> MISYDNYVTILDEETLKAWIAKLEKAPVFAFDTETDSLDNISANLVGLSFAIEPGVAAYIPVAHDYLDAPDQISRERALELLKPLLEDEKALKVGQNLKYDRGILANYGIELRGIAFDTMLESYILNSVAGRHDMDSLAERWLKHKTITFEEIAGKGKNQLTFNQIALEEAGRYAAEDADVTLQLHLKMWPDLQKHKGPLNVFENIEMPLVPVLSRIERNGVKIDPKVLHNHSEELTLRLAELEKKAHEIAGEEFNLSSTKQLQTILFEKQGIKPLKKTPGGAPSTSEEVLEELALDYPLPKVILEYRGLAKLKSTYTDKLPLMINPKTGRVHTSYHQAVTATGRLSSTDPNLQNIPVRNEEGRRIRQAFIAPEDYVIVSADYSQIELRIMAHLSRDKGLLTAFAEGKDIHRATAAEVFGLPLETVTSEQRRSAKAINFGLIYGMSAFGLARQLNIPRKEAQKYMDLYFERYPGVLEYMERTRAQAK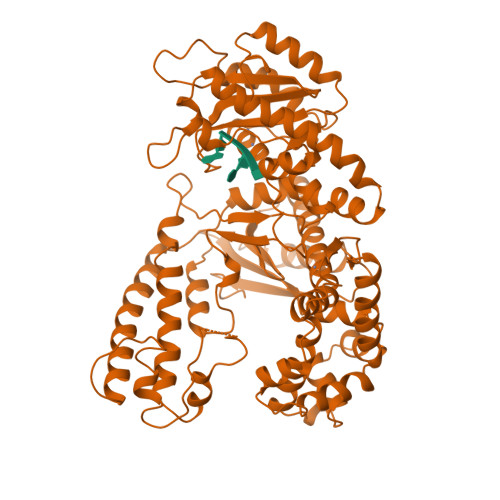EQGYVETLDGRRLYLPDIKSSNGARRAAAERAAINAPMQGTAADIIKRAMIAVDAWLQAEQPRVRMIMQVHDELVFEVHKDDVDAVAKQIHQLMENCTRLDVPLLVEVGSGENWDQAH> KEVCYERLGCFSDDSPWSGITERPLHILPWSPKDVNTRFLLYTNENPNNFQEVAADSSSISGSNFKTNRKTRFIIHGFIDKGEENWLANVCKNLFKVESVNCICVDWKGGSRTGYTQASQNIRIVGAEVAYFVEFLQSAFGYSPSNVHVIGHSLGAHAAGEAGRRTNGTIGRITGLDPAEPCFQGTPELVRLDPSDAKFVDVIHTDGAPIVPNLGFGMSQVVGHLDFFPNGGVEMPGCKKNILSQIVDIDGIWEGTRDFAACNHLRSYKYYTDSIVNPDGFAGFPCASYNVFTANKCFPCPSGGCPQMGHYADRYPGKT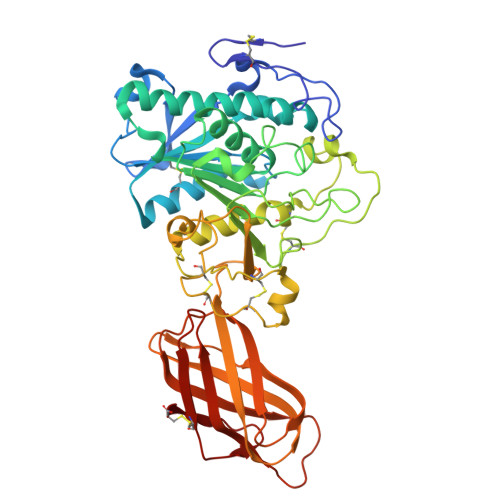NDVGQKFYLDTGDASNFARWRYKVSVTLSGKKVTGHILVSLFGNKGNSKQYEIFKGTLKPDSTHSNEFDSDVDVGDLQMVKFIWYNNVINPTLPRVGASKIIVETNVGKQFNFCSPETVREEVLLTLTPC>[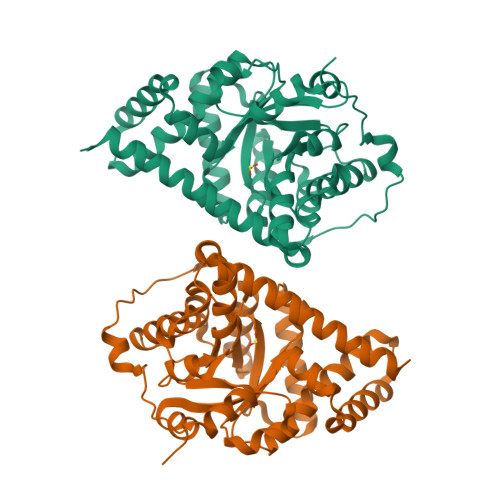2x]GSSGSSGMESALDQLKQFTTVVADTGDFNAIDEYKPQDATTNPSLILAAAQMPAYQELVEEAIAYGKKLGGPQEEQIKNAIDKLFVLFGAEILKKIPGRVSTEVDARLSFDKDAMVARARRLIELYKEAGVGKDRILIKLSSTWEGIQAGKELEEQHGIHCNMTLLFSFAQAVACAEAGVTLISPFVGRILDWHVANTDKKSYEPQGDPGVKSVTKIYNYYKKFGYKTIVMGASFRNTGEIKALAGCDFLTISPKLLGELLKDNSKLAPALSVKAAQTSDSEKIHLDEKAFRWLHNEDQMAVEKLSDGIRKFAADAIKLERMLTERMFSAE>[2x]NSINDSKILSLQNK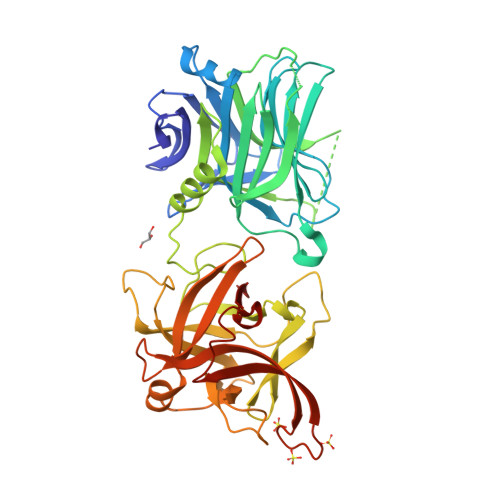KNTLMDTSGYNAEVRVEGNVQLNPIFPFDFKLGSSGDDRGKVIVTQNENIVYNAMYESFSISFWIRINKWVSNLPGYTIIDSVKNNSGWSIGIISNFLVFTLKQNENSEQDINFSYDISKNAAGYNKWFFVTITTNMMGNMMIYINGKLIDTIKVKELTGINFSKTITFQMNKIPNTGLITSDSDNINMWIRDFYIFAKELDDKDINILFNSLQYTNVVKDYWGNDLRYDKEYYMINVNYMNRYMSKKGNGIVFNTRKNNNDFNEGYKIIIKRIRGNTNDTRVRGENVLYFNTTIDNKQYSLGMYKPSRNLGTDLVPLGALDQPMDEIRKYGSFIIQPCNTFDYYASQLFLSSNATTNRLGILSIGSYSFRLGGDWYRHEYLIPVIKIEHYASLLESTSTHWVFVPASE> STTEVVMENVTAFWEEGFGELLEKAKQNNNNRKTSNGDDSLSFSNLSLLGTPVLKDINFKIERGQLLAVAGSTGAG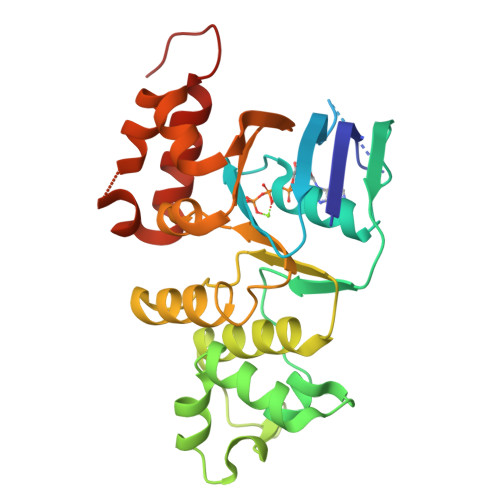KTSLLMMIMGELEPSEGKIKHSGRISFCSQFSWIMPGTIKENIIGVSYDEYRYRSVIKACQLEEDISKFAEKDNIVLGEGGITLSEGQQAKISLARAVYKDADLYLLDSPFGYLDVLTEKEIFESCVCKLMANKTRILVTSKMEHLKKADKILILHEGSSYFYGTFSELQNLQPDFSSKLMGCDSFDQFSAERRNSILTETLRRFSLEGDAPVS>[2x]MHRTSNGSHATGGNLPDVASHYPVAYEQTLDGTVGFVIDEMTPERATASVEVTDTLRQRWGLVHGGAYCALAEMLAAEATVAVVHEKGMMAVGQ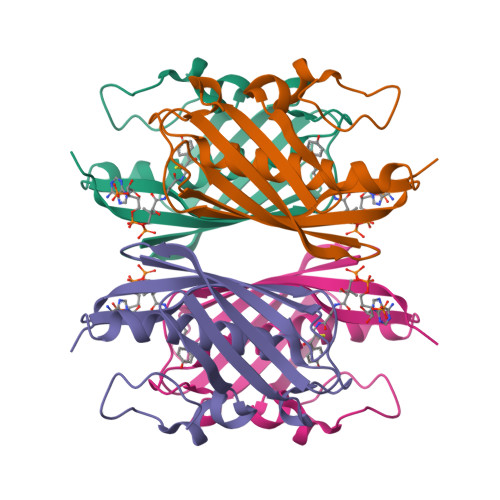SNHTSFFRPVKEGHVRAEAVRIHAGSTTWFWDVSLRDDAGRLCAVSSMSIAVRPRRD>MNSTENKNFVISISTAEQRRNHIIEQFTHQNIPFEFFDAFTPSDKLTDHLQRYLPNVANAAQLTMGEKGCLMSHFMLWKKCIDENLDYITLFEDDILLGENANKFLAEGDWLKVRFNFQEIFVLRLETFLMPVQLEKQTQIPPFQQRDIDILTSKHFGTAGYVISQGAAKYLIALFEK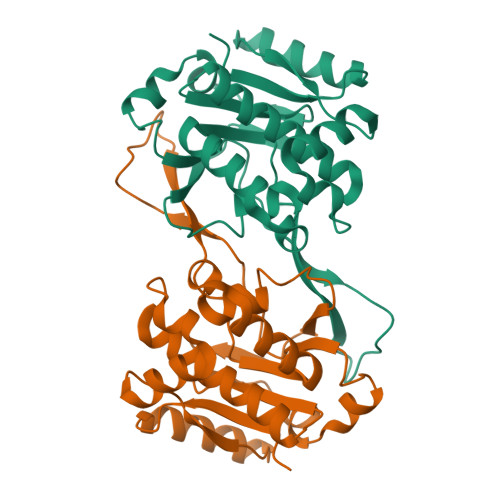LTTEEIKPIDEIMFNQQINATDYRVYQLNPAICVQELQLNQEASLLVSNLEQERKINLKYEKRKHLEHHHHHH[2x]> MITCRDIITLGLQQARVVPLGREPKAKEADAGLTVLQSIYDSMFADGPLGPFTEVYATSAYTAQENERI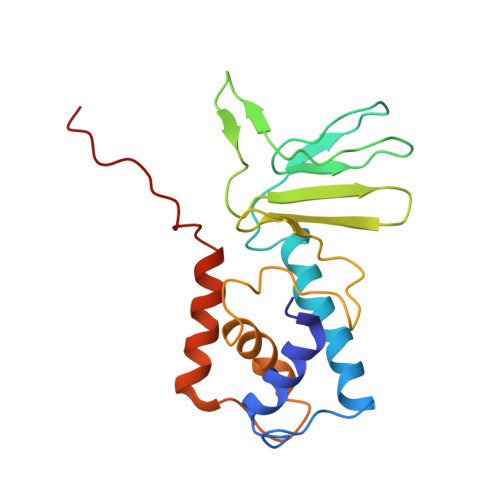VTNGAAITIPQTITEGNETRKPYDLTAIIVINGAAQENHVFSLGRWQTAHDLTLNSEAPLAERDKAGLAALFAMEFAEMFGAELPPRTTARGFRFKGAISQKLATKRDDPVYY>LPSGSDPAFSQPKSVLDAGLTCQGASPSSVSKPILLVPGTGTTGPQSFDSNWIPLSTQLGYTPCWISPPPFMLNDTQVNTEYMVNAITALYAGSGNNKLPVLTWSQGGLVAQWGLTFFPSIRSKVDRLMAFAPDYKGTVLAGPLDALAVSAPSVWQQTTGSALTTALRNAGGLTQIVPTTNLYSATDEIVQPQVSNSPLDSSYLFNGKNVQAQAVCGPLFVIDHAGSLTSQFSYVVGRSALRSTTGQARSADYGIT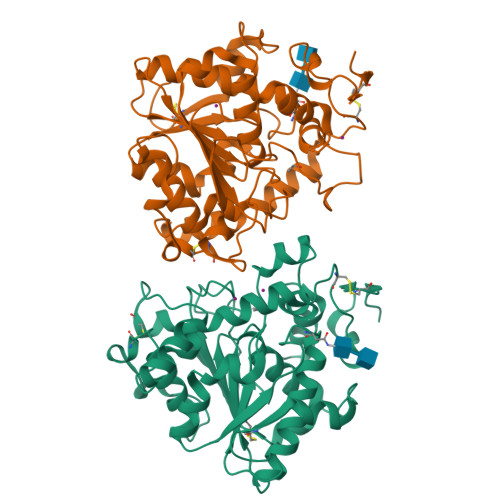DCNPLPANDLTPEQKVAAAALLAPAAAAIVAGPKQNCEPDLMPYARPFAVGKRTCSGIVTP[2x]>[2x]SSSSTASASAKKIIVKHVTVIGGGLMGAGIAQVAAATGHTVVLVDQTEDILAKSKKGIEESLRKVAKKKFAENPKAGDEFVEKTLSTIATSTDAASVVHSTDLVVEAIVENLKVKN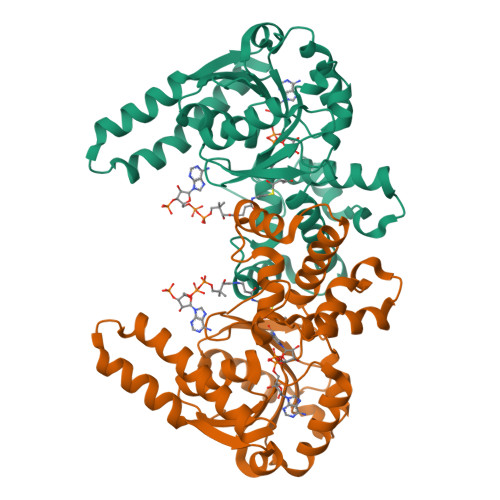ELFKRLDKFAAEHTIFASNTCSLQITSIANATTRQDRFAGLHFFNPVPVMKLVEVIKTPMTSQKTFESLVDFSKALGKHPVSCKDTPGFIVNRLLVPYLMEAIRLYERGDASKEDIDTAMKLGAGYPMGPFELLDYVGLDTTKFIVDGWHEMDAENPLHQPSPSLNKLVAENKFGKKTGEGFYKYK C. perfringens type G, the causative agent of necrotic enteritis in broilers, produces two glycosyl hydrolase family 18 chitinases, ChiA and ChiB, which display distinct substrate preferences. Whereas ChiB preferentially processes linear substrates such as chitin, ChiA prefers larger and more branched substrates, such as carbohydrates presented by the chicken intestinal mucus. Here, we show via crystal structures of ChiA and ChiB in the apo and ligand-bound forms that the two enzymes display structural features that explain their substrate preferences providing a structural blueprint for further interrogation of their function and inhibition. We succeeded in obtaining several crystal structures of recombinant ChiA and ChiB in apo (unbound) and ligand-bound forms to resolutions between 1.30 Å and 1.85 Å. Both ChiA and ChiB encode for an N-terminal glycosyl hydrolase family 18 (GH18) Trios-phosphate Isomerase (TIM) barrel followed by a C-terminal putative carbohydrate binding domain (CBD).

The -2 and -1 positions, where the product disaccharide is bound, are also the location where the inhibitor Bisdionin C binds. The inhibitor molecule forces D194 into its resting conformation where it engages D192 in a low-barrier hydrogen bond as the other conformation would cause steric clashes. A second low occupancy or highly disordered Bisdionin C molecule might be bound in the vicinity of W257, more towards the CBD. Bisdionin C is known to target bacterial GH18 enzymes but could result in unspecific targeting.

> MGSSELNRKLVGYFPEWAYSSEAQGYFNVTDLQWDSLTHIQYSFAMVDPSTNKITLSNKHAAIEEDFSEFDLNYNGKKIELDPSLPYKGHFNVLQTMKKNYPDVSLLISVGGWTGTRCFYTMIDTDNRINTFADSCVDFIRKYGFDGVDIDFEYPSSTSQSGNPDDFDLSEPRRTKLNERYNILIKTLREKIDMASKEDGKEYLLTAAVTASPWVLGGISDNTYAKYLDFLSIMSYDYHGGWNEYVEHLAGIYPNKEDRETVTQIMPTLCMDWAYRYYRGVLPAEKILMGIPYYTRGWENVQGGINGLHGSSKTPASGKYNILGDDLNNDGVLEPAGANPLWHVLNLMEQDPNLKVYWDEISKVPYVWQNDKKVFVSFENEKSIDARLEYIQNKNLGGALIWVMNGDYGLNPNYVEGSNKINEGKYTFGDTLTKRLSQGLKKMGVCNKTPDDLNISLEPINVDVKFNGKYDHPNYTYSIDITNYTDKEIKGGWNVSFDLPKSAVFKSSWGGTYSVTDNGDFNTITLTSGAWQNIAPNSTITVQGMIGLCFSGIRNVTFNGMNPIGNDKSHHHHHH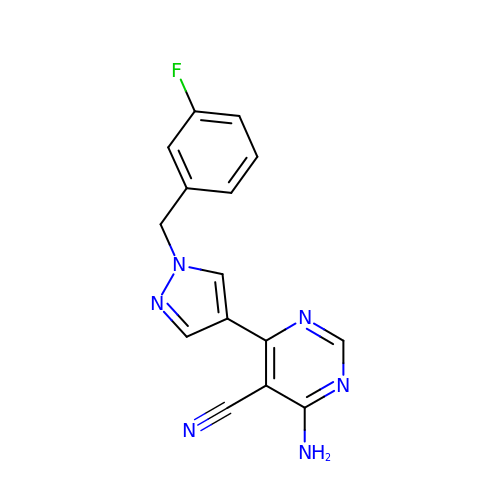4-azanyl-6-[1-[(3-fluorophenyl)methyl]pyrazol-4-yl]pyrimidine-5-carbonitrile | C15 H11 F N6 | VYNWCICHANBKCE-UHFFFAOYSA-N N-(4-{[(4S)-3-amino[1,2,4]triazolo[4,3-b]pyridazin-6-yl]sulfanyl}phenyl)acetamide | C13 H12 N6 O S | 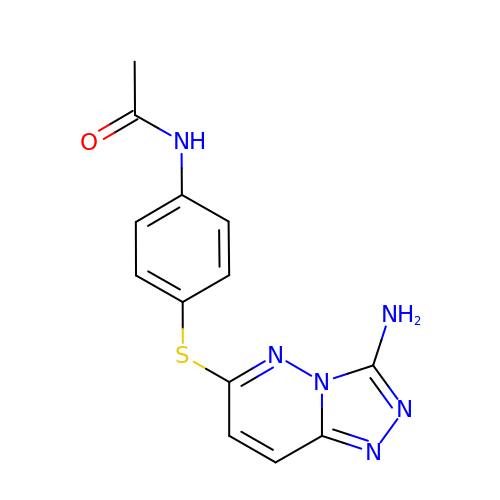DDVAGHQEXKJINC-UHFFFAOYSA-N>[2x]EVSAEEIKKHEEKWNK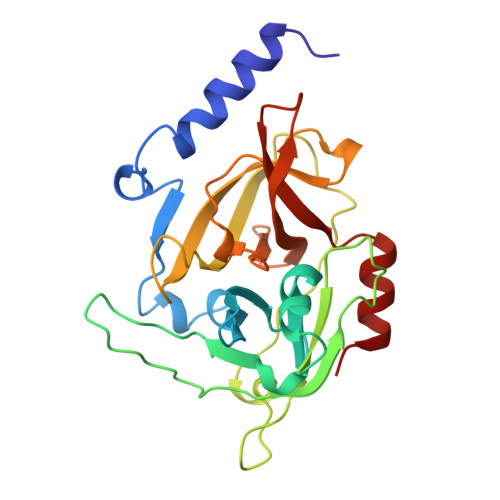YYGVNAFNLPKELFSKVDEKDRQKYPYNTIGNVFVKGQTSATGVLIGKNTVLTNRHIAKFANGDPSKVSFRPSINTDDNGNTETPYGEYEVKEILQEPFGAGVDLALIRLKPDQNGVSLGDKISPAKIGTSNDLKDGDKLELIGYPFDHKVNQMHRSEIELTTLSRGLRYYGFTVPGNSGSGIFNSNGELVGIHSSKVSHLDREHQINYGVGIGNYVKRIINEKNE>AKVNLYISNDAYEKINAIIEKRRQEGAREKDVSFSATASMLLELGLRVHEA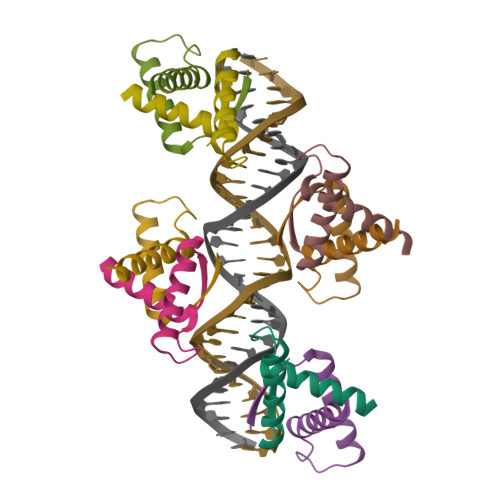QM[8x]> GLTCVTSKSIFGITTEDCPDGQNLCFKRRHYVVPAIYDSTRGCAATCPIPENYDSIHCCK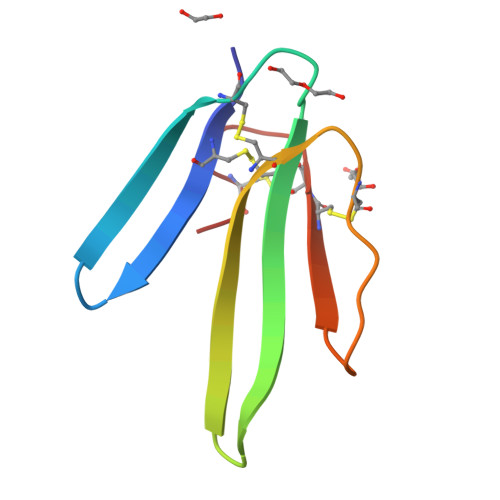TDKCNE>GMAPPSVFAEVPQAQPVLVFKLIADFREDPDPRKVNLGVGAYRTDDCQPWVLPVVRKVEQRIANNSSLNHEYLPILGLAEFRTCASRLALGDDSPALQEKRVGGVQSLGGTGALRIGAEFLARWYNGTNNKDTPVYVSSPTWENHNGVFTTAGFKDIRSYRYWDTEKRGLDLQGFLSDLENAPEFSIFVLHACAHNPTGTDPTPEQWKQIASVMKRRFLFPFFDSAYQGFASGNLEKDAWAIRYFVSEGFELFCAQSFSKNFGLYNERVGNLTVVAKEPDSILRVLSQMQKIVRVTWSNPPAQGARIVART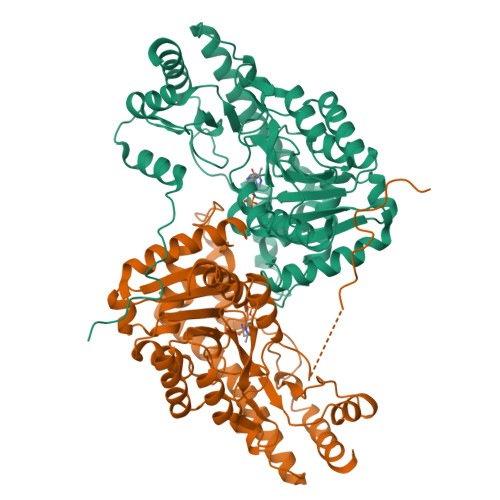LSDPELFHEWTGNVKTMADRILSMRSELRARLEALKTPGTWNHITDQIGMFSFTGLNPKQVEYLINQKHIYLLPSGRINMCGLTTKNLDYVATSIHEAVTKIQ[2x]The most abundant group of viruses, comprising tailed bacteriophages and evolutionarily related herpesviruses, specifically recognize their genomic DNA and package it into a preformed shell (capsid). The key component ensuring specific recognition of viral DNA from the mixture of all the nucleic acids contained in the host cell, and initiating its packaging is the small terminase protein. Packaging initiation occurs when the small terminase binds to a specific sequence (pac or cos) in the genomic DNA, facilitating the cleavage of the dsDNA by large terminase and subsequent assembly of the large terminase bound DNA complex onto the portal protein vertex of the capsid for packaging to begin. All small terminase structures broadly resemble each other in architecture, with 8 to 12 protomers oligomerized in a ring to form a central channel in the middle, with the N-terminal segments arrayed around the outside.

The complex of small terminase with the longest of these fragments was purified from unbound DNA using size exclusion chromatography and the structure of this complex was determined at a resolution of 3.0 Å by cryoEM. In the complex, DNA is threaded through the central channel, bent toward one side of the small terminase nonamer to form an asymmetric complex. Strikingly, in the small terminase:DNA complex, density for the N-terminal residues Asp3-Val23 of one protomer and the C terminus—residues Gly125 to Asp145—of the adjacent protomer is clearly resolved in the map. The N terminus of one protomer and the C terminus of the adjacent protomer each form an α-helix that pack against each other, in a manner reminiscent to that in a classical HTH motif, to create a DNA-binding substructure. The orientation of these two helices is stabilized by 6 interhelix hydrogen bonds and the buried surface area between the helices is 430 Å2. These helices form a scaffold that places the N-terminal arm (NTA) of the N-terminal helix in the minor groove, while the end of the C-terminal helix is inserted into the major groove where the DNA is bent as it exits the central channel. Four rings of lysine and arginine residues: Lys96, Lys100, Arg107, and Arg114 line the channel and form hydrogen bonds with phosphates of the DNA backbone. Direct hydrogen-bonding interactions of small terminase with bases of DNA are formed solely by the DNA-binding substructure. Arg128 forms bidentate hydrogen bonds with the base of G at position 21 in the center of the small terminase binding site. Arg7 forms bifurcated hydrogen bonds with T16 at the 5′ end of the small terminase binding site (in the top strand). The DNA is bent to an angle of 34° at the point at which Arg128 forms hydrogen bonds with G at position 21.

>MADKRIRSDSSAAAVQAMKNAAVDTIDPPSHAGLEKKAEPFWHDNIRSKALDSWTPADLLAAVELANNQLYITVLRKDLRKEERIRGEERDEGLIKDLRKQIVELQRTILAQRRDLQIHSHATNGESRDQKKRNQNDRDARNTKNEHQDQDDNLIAFPKHG[9x]>[2x]GSSHHHHHHSSGLVPRGSMSTSWSDRLQNAADMPANMDKHALKKYRREAYHRVFVNRSLAMEKIKCFGFNMDYTLAVYKSPEYESLGFELTVERLVSIGYPQELLSFAYDSTFPTRGLVFDTLYGNLLKVDAYGNLLVCAHGFNFIRGPETREQYPNKFIQRDDTERFYILNTLFNLPETYLLACLVDFFTNCPRYTSCETGFKDGDLFMSYRSMFQDVRDAVDWVHYKGSLKEKTVENLEKYVVKDGKLPLLLSRMKEVGKVFLATNSDYKYTDKIMTYLFDFPHGPKPGSSHRPWQSYFDLILVDARKPLFFGEGTVLRQVDTKTGKLKIGTYTGPL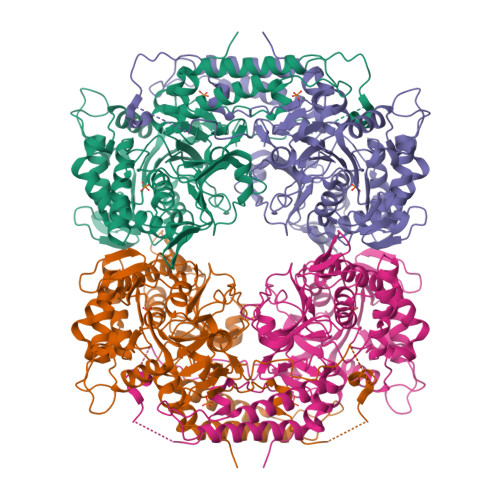QHGIVYSGGSSDTICDLLGAKGKDILYIGDHIFGDILKSKKRQGWRTFLVIPELAQELHVWTDKSSLFEELQSLDIFLAELYKHLDSSSNERPDISSIQRRIKKVTHDMDMCYGMMGSLFRSGSRQTLFASQVMRYADLYAASFINLLYYPFSYLFRAAHVLMPHESTVEHTHVDINEMESPLATRNRTSVDFKDTDYKRHQLTRSISEIKPPNLFPLAPQEITHCHDEDDDEEEEEEEE>DRHHHHHHGSEVVVEWSRDQYHVLFDSYRDNVAGKSFQTRLCLPMPIDVVYTWVNGTDPKLIKEVTELKRSKRDPLIPECQGKQTPEKDKCYRDDNTASRFEDNEELRYSLRSIEKHAPWVRHIFIVTNGQIPSWLNLDNPRVSVVTHQDIFQNQTHLPTFSSPAIETHIHRIPGLSQKFIYLNDDVMFGKDVWPDDFYSHSKGQKVYLTWPVPNDTFADSLRYVNRLLNAQFGFTSRKVPAHMPHMIDRLIMQELQDTFPQEFDKTSSHRVRHSEDMQFAFSYFYFLMSAVQQLNISEVFDEIDTDHSGVLSDREIRTLATRIHELPLSLQDLTSLEQMLINCSKSLPSNLTHLHAVSPTQEAYYDPSMPPVTKGLVIHCKPITERIHKAFKDQNKYKFEIMGEEEIAFKMIRTNV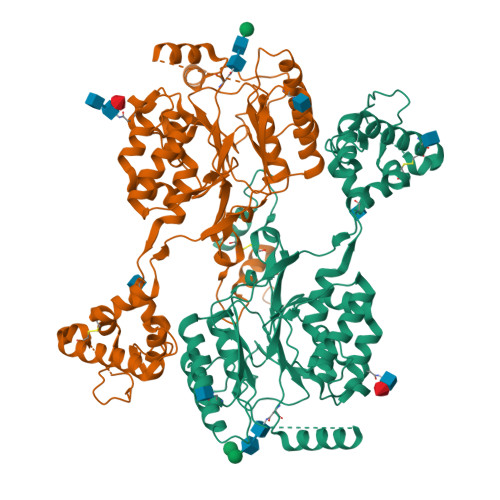SHVVGQLDDIRKNPRKFICLNDNIDHIHKDAGTVKAVLRDFYESMFPLPSQFELPREYRNRFLHMTELQEWRIYRDKL[2x]> MAYSYTEKKRIRKDFSKLPDVMDVPYLLAIQLDSYREFLQAGATKEQFRDVGLHAAFKSVFPIISYSGNAALEYVGYRLGEPAFDVKECVLRGVTFAVPLRVKVRLIIFDRESSNKAIKDIKEQEVYMGEIPLMTENGTFIINGTERVIVSQLHRSPGVFFDHDRGKTHSSGKLLYSARIIPYRGSWLDFEFDPKDCVFVRIDRRRKLPASVLLRALGYSTEEILNAFYATNVFHIKGETLNLELVPQRLRGEVASIDIKDGSGKVIVEQGRRITARHINQLEKAGVSQLEVPFDYLIGRTIAKAIVHPATGEIIAECNTELTLDLLAKVAKAQVVRIETLYTNDIDCGPFISDTLKIDNTSNQLEALVEIYRMMRPGEPPTKEAAETLFGNLFFSAERYDLSAVGRMKFNRRIGRTEIEGPGVLSKEDIIDVLKTLVDIRNGKGIVDDIDHLGNRRVRCVGEMAENQFRVGLVRVERAVKERLSMAESEGLMPQDLINAKPVAAAIKEFFGSSQLSQFMDQNNPLSEITHKRRVSALGPGGLTRERAGFEVRDVHPTHYGRVCPIETPEGPNIGLINSLATYARTNKYGFLESPYRVVKDSLVTDEIVFLSAIEEADHVIAQASATLNEKGQLVDELVAVRHLNEFTVKAPEDVTLMDVSPKQVVSVAASLIPFLEHDDANRALMGSNMQRQAVPTLRADKPLVGTGMERNVARDSGVCVVARRGGVIDSVDASRVVVRVADDEVETGEAGVDIYNLTKYTRSNQNTCINQRPLVSKGDVVARGDILADGPSTDMGELALGQNMRVAFMPWNGFNFEDSICLSERVVQEDRFTTIHIQELTCVARDTKLGPEEITADIPNVGEAALNKLDEAGIVYVGAEVQAGDILVGKVTPKGETQLTPEEKLLRAIFGEKASDVKDTSLRVPTGTKGTVIDVQVFTRDGVERDSRALSIEKMQLDQIRKDLNEEFRIVEGATFERLRAALVGAKAEGGPALKKGTEITDDYLDGLERGQWFKLRMADDALNEQLEKAQAYISDRRQLLDDKFEDKKRKLQ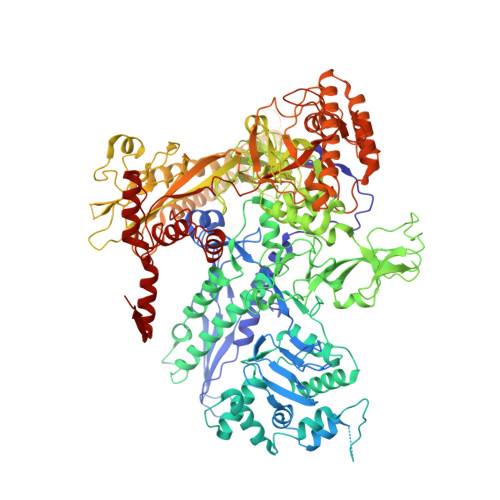QGDDLAPGVLKIVKVYLAIKRRIQPGDKMAGRHGNKGVVSVIMPVEDMPHDANGTPVDIVLNPLGVPSRMNVGQILETHLGLAAKGLGEKINRMLEEQRKVAELRKFLHEIYNEIGGREENLDELGDNEILALAKNLRGGVPMATPVFDGAKEREIKAMLKLADLPESGQMRLFDGRTGNQFERPTTVGYMYMLKLNHLVDDKMHARSTGSYSLVTQQPLGGKAQFGGQRFGEMEVWALEAYGAAYTLQEMLTVKSDDVNGRTKMYKNIVDGDHRMEAGMPESFNVLIKEIRSLGIDIELETE> GSSST;> GLGQMLESMIDNTVRETVGAATSRDALPNTEASGPTHSK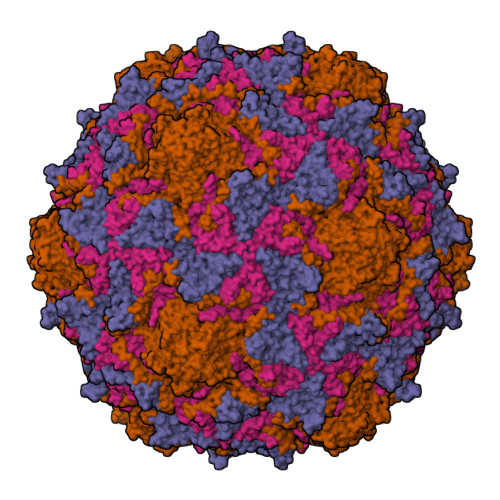EIPALTAVETGATNPLVPSDTVQTRHVVQHRSRSESSIESFFARGACVTIMTVDNPASTTNKDKLFAVWKITYKDTVQLRRKLEFFTYSRFDMELTFVVTANFTETNNGHALNQVYQIMYIPPGAPVPEKWDDYTWQTSSNPSIFYTYGTAPARISVPYVGISNAYSHFYDGFSKVPLKDQSAALGDSLYGAASLNDFGILAVRVVNDHNPTKVTSKIRVYLKPKHIRVWCPRPPRAVAYYGPGVDYKDGTLTPLSTKDLTTY;> SPNIEACGYSDRVLQLTLGNSTITTQEAANSVVAYGRWPEYLRDSEANPVDQPTEPDVAACRFYTLDTVSWTKESRGWWWKLPDALRDMGLFGQNMYYHYLGRSGYTVHVQCNASKFHQGALGVFAVPEMCLAGDSNTTTMHTSYQNANPGEKGGTFTGTFTPDNNQTSPARRFCPVDYLLGNGTLLGNAFVFPHQIINLRTNNCATLVLPYVNSLSIDSMVKHNNWGIAILPLAPLNFASESSPEIPITLTIAPMCCEFNGLRNITLPRLQ;> GLPVMNTPGSNQYLTADNFQSPCALPEFDVTPPIDIPGEVKNMMELAEIDTMIPFDLSATKKNTMEMYRVRLSDKPHTDDPILCLSLSPASDPRLSHTMLGEILNYYTHWAGSLKFTFLFCGSMMATGKLLVSYAPPGADPPKKRKEAMLGTHVIWDIGLQSSCTMVVPWISNTTYRQTIDDSFTEGGYISVFYQTRIVVPLSTPREMDILGFVSACNDFSVRLLRDTTHIEQKALAQ;> GAQVSSQKVGAHENSNRAYGGSTINYTTINYYRDSASNAASKQDFSQDPSKFTEPIKDVLIKTAPMLN> MGSSHHHHHHGSGENLYFQSNQPLKIVVPFSAGGTADVLPRLVAEKIRADYAGGVIIENKPGAGGNIGADLVFRAPPDGMTVLASPPGPIAINHNLYQKLSFDPTRWVPVTILATVPNVLVINPKLPVKSLGEFIAYAKANPKKVTVATQGDGSTSHLTAAMFMQLTGTELTVIPYKGTAPALIDLIGGNVDVFFDNISSSATYHQAGKVRILAVADEQRSQILPQVPTFAEQQWPAMQAVTFFSVVAPPGTSAEIAQKLQKQMALALS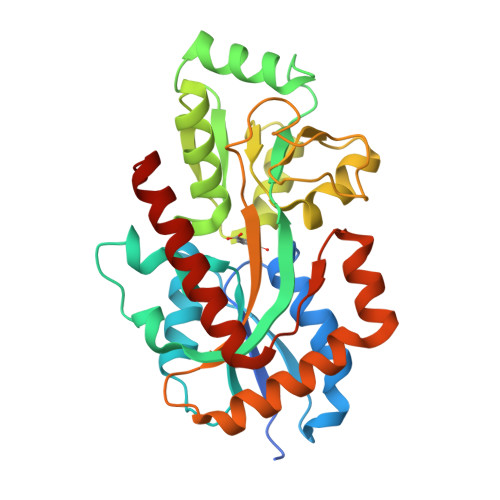SNDIRKHFQEQGAVPCGWDPSKTAQFIRQETEKWKKVLKAANVKL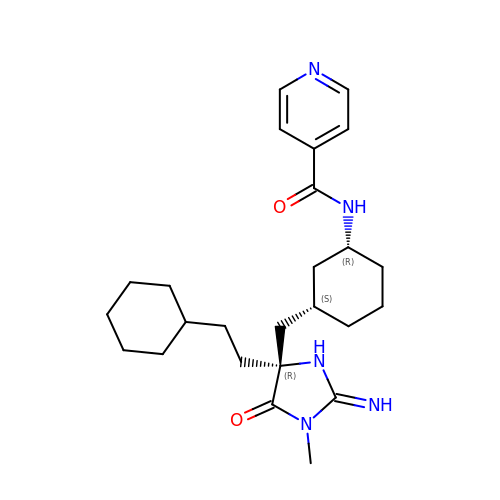N-[(1R,3S)-3-{[(2E,4R)-4-(2-cyclohexylethyl)-2-imino-1-methyl-5-oxoimidazolidin-4-yl]methyl}cyclohexyl]pyridine-4-carboxamide | C25 H37 N5 O2 | NAGJGYNUXJYJOV-PIBDYAPNSA-N> MSAYATQGFNLDDRGRRIVVDPVTRIEGHMRCEVNVDANNVIRNAVSTGTMWRGLEVILKGRDPRDAWAFVERICGVCTGCHALASVRAVENALDIRIPKNAHLIREIMAKTLQVHDHAVHFYHLHALDWVDVMSALKADPKRTSELQQLVSPAHPLSSAGYFRDIQNRLKRFVESGQLGPFMNGYWGSKAYVLPPEANLMAVTHYLEALDLQKEWVKIHTIFGGKNPHPNYLVGGVPCAINLDGIGAASAPVNMERLSFVKAR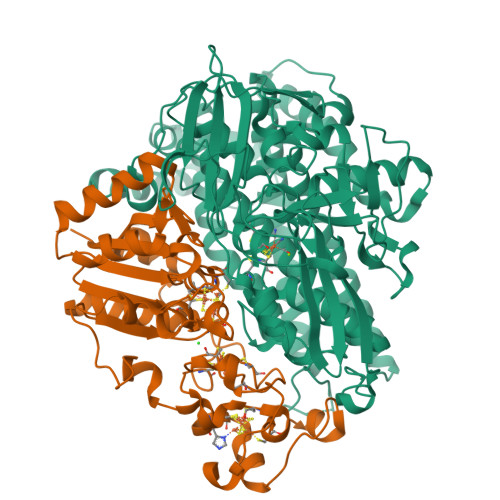IDEIIEFNKNVYVPDVLAIGTLYKQAGWLYGGGLAATNVLDYGEYPNVAYNKSTDQLPGGAILNGNWDEVFPVDPRDSQQVQEFVSHSWYKYADESVGLHPWDGVTEPNYVLGANTKGTRTRIEQIDESAKYSWIKSPRWRGHAMEVGPLSRYILAYAHARSGNKYAERPKEQLEYSAQMINSAIPKALGLPETQYTLKQLLPSTIGRTLARALESQYCGEMMHSDWHDLVANIRAGDTATANVDKWDPATWPLQAKGVGTVAAPRGALGHWIRIKDGRIENYQCVVPTTWNGSPRDYKGQIGAFEASLMNTPMVNPEQPVEILRTLHSFDPCLACSTH;> METKPRTPVLWLHGLECTCCSESFIRSAHPLAKDVVLSMISLDYDDTLMAAAGHQAEAILEEIMTKYKGNYILAVEGNPPLNQDGMSCIIGGRPFIEQLKYVAKDAKAIISWGSCASWGCVQAAKPNPTQATPVHKVITDKPIIKVPGCPPIAEVMTGVITYMLTFDRIPELDRQGRPKMFYSQRIHDKCYRRPHFDAGQFVEEWDDESARKGFCLYKMGCKGPTTYNACSTTRWNEGTSFCIQSGHGCIGCSEDGFWDKGSFYDRLTGISQFGVEANADKIGGTASVVVGAAVTAHAAASAIKRASKKNETSGSEHRSAWSHPQFEK>GSMASLPVLQKESVFQSGAHAYRIPALLYLPGQQSLLAFAEQRASKKDEHAELIVLRRGDYDAPTHQVQWQAQEVVAQARLDGHRSMNPCPLYDAQTGTLFLFFIAIPGQVTQQQQLQTRANVTRLCQVTSTDHGRTWSSPRDLTDAAIGP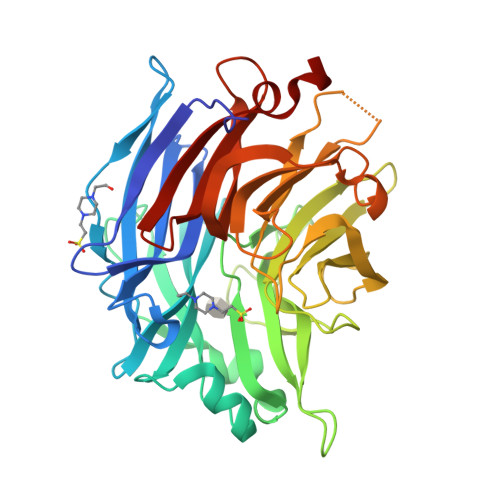AYREWSTFAVGPGHCLQLNDRARSLVVPAYAYRKLHPIQRPIPSAFCFLSHDHGRTWARGHFVAQDTLECQVAEVETGEQRVVTLNARSHLRARVQAQSTNDGLDFQESQLVKKLVEPPPQGCQGSVISFPSPRSGPGSPAQWLLYTHPTHSWQRADLGAYLNPRPPAPEAWSEPVLLAKGSCAYSDLQSMGTGPDGSPLFGCLYEANDYEEIVFLMFTLKQAFPAEYLPQ[2x]Many bacterial and eukaryotic viruses with double-stranded DNA genomes in the realms Duplodnaviria and Varidnaviria encode homologs of cellular RNAPs (collectively denoted “two-barrel RNAPs”). The TMP-fused virion RNAP transcribes pre-early phage genes, including a gene that encodes another, non-virion RNAP, that transcribes early and some middle phage genes. Transcription by vRNAP and nvRNAP is directed by dissimilar AT-rich and GC-rich promoters, respectively, and the two phage RNAPs have distinct overall architectures, with the TMP-fused vRNAP being unusually flat and lacking the clamp domain.

Gp64 is a non-virion RNAP (nvRNAP) that may transcribe phage genes at later stages of infection. Heterologously produced gp64 also extended the RNA component of the scaffold in a template-dependent manner. The crystal structures of gp64 nvRNAP and one of its close homologs (gp62 of phage P74-26) were also determined at 2.7 Å and 2.4 Å resolution, respectively, and found to be essentially identical. The overall architectures of gp96 vRNAP and gp64 nvRNAP are markedly different. The gp64 nvRNAP structure resembles the structures of other two-barrel RNAPs and has a characteristic crab-claw-like architecture that includes the clamp domain. The non-virion RNAP has a crab-claw-like architecture. Gp64 is distributed along a much larger, 49 kbp region extending from the left end to the middle part of the genome (genes 1-77) and thus interacts not only with early but also with middle phage genes. The pre-early genes include the gene encoding nvRNAP gp64, which transcribes the early and some middle genes of the phage. We therefore propose that these motifs define phage promoters; gp96 vRNAP initiates transcription at the AT-rich promoters, whereas gp64 nvRNAP initiates transcription at the GC-rich promoters.

>[2x]MGTERIGTLLGWNLLEFPKERVRELQSTAEPTEGSYRNILDGLVNLVKEALGHIPDALIGKDNVVMWPGSTGANFHLPGWRVSDFVRAPSRARTELPTSSLTLIRGKKVFGDGIVGIFPPMPEIVPSPNGWAQVRMFSRRGNEIFRAWKGVIVTHPNVKEPLVAFDDGYGVEELGDVLEIHAILLQTQFTAEYTVQGLYYQGIPGWWRYLDLDFAFPPDKAKLVEAGAPLELLYPIAQYLKLKGPNTGFGGILLSPKILPFLGLHGLEDGGLLAYTRRWRPGERVIFNRRPDLPTGQSAVELTYLGLSPIADSVIAHEGDIASTGADYDGDIGYLFPTPEKGGLYMPFHGEALHRKDLPTKDYESGLHRWAGQVHAAHILGRVEVNTRRLLDVAWANGEDVPQDYLHAATEMIQVAVDRQKRDIQWPDFDFKSVKDPVMTDFWRLAVPGGKLTPEGNTPAAKITNRWRAWETLDGYVGHPHMKNDLKPLASKISRVLARGEHRRPGPVLAALAFALLAPEPRPKEVEDLLTAGLQSGKRHAVYDALVQMGLPANQATDHPELWLRLASKEELEAIFKQLGYRPAMEELEEALNAVDGMDTSANRAPLDTLFADLFRV8-[3-(3-azanyl-2~{H}-indazol-6-yl)-5-chloranyl-pyridin-4-yl]-2,8-diazaspiro[4.5]decan-1-one | C20 H21 Cl 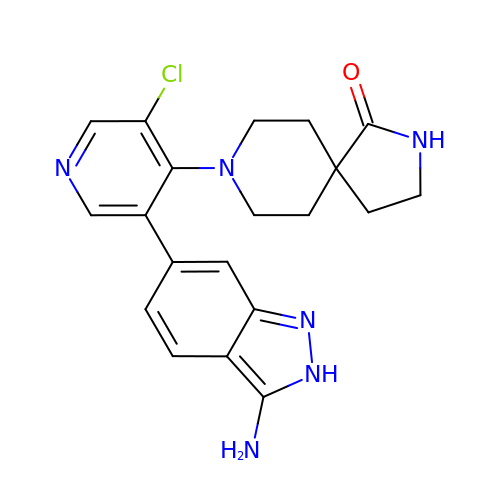N6 O | ZVSGCPGPQNLKLU-UHFFFAOYSA-N> EFMVSLPRMVYPQPKVLTPCRKDVLVVTPWLAPIVWEGTFNIDILNEQFRLQNTTIGLTVFAIKKYVAFLKLFLETAEKHFMVGHRVHYYVFTDQPAAVPRVTLGTGRQLSVLEVGAYKRWQDVSMRRMEMISDFCERRFLSEVDYLVCVDVDMEFRDHVGVEI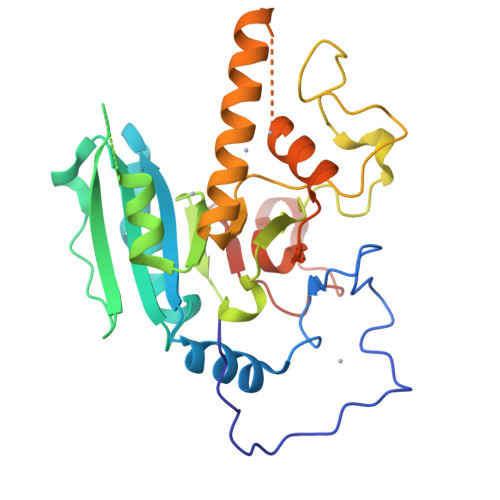LTPLFGTLHPSFYGSSREAFTYERRPQSQAYIPKDEGDFYYMGAFFGGSVQEVQRLTRACHQAMMVDQANGIEAVWHDDSHLNKYLLRHKPTKVLSPEYLWDQQLLGWPAVLRKLRFTAVPKNHQAVRNPE>MPLLLLLPLLWAGALAELHHHHHHENLYFQSGRYKCGISKACPEKHFAFKMASGAANVVGPKICLEDNVLMSGVKNNVGRGINVALANGKTGEVLDTKYFDMWGGDVAPFIEFLKAIQDGTIVLMGTYDDGATKLNDEARRLIADLGSTSITNLGFRDNWVFCG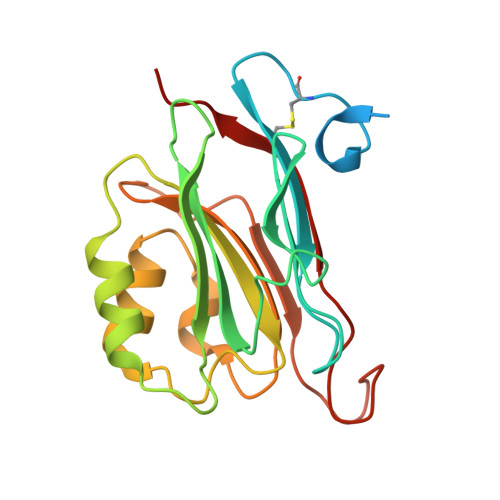GKGIKTKSPFEQHIKNNKDTNKYEGWPEVVEMEGCIPQKQD[2x]> DHSLEAQWTKWKAMHNRLYGMNEEGWRRAVWEK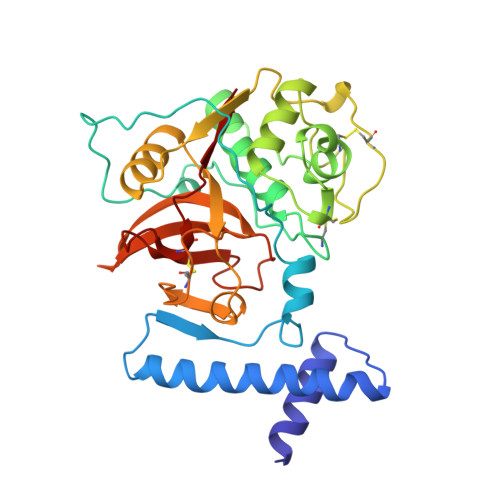NMKMIELHNQEYREGKHSFTMAMNAFGDMTSEEFRQVMNGLQNRKPRKGKVFQEPLFYEAPRSVDWREKGYVTPVKNQGQCGSSWAFSATGALEGQMFRKTGRLISLSEQNLVDCSGPEGNEGCNGGLMDYAFQYVQDNGGLDSEESYPYEATEESCKYNPKYSVANDAGFVDIPKQEKALMKAVATVGPISVAIDAGHESFLFYKEGIYFEPDCSSEDMDHGVLVVGYGFESTESDGNKYWLVKNSWGEEWGMGGYVKMAKDRRNHCGIASAASYPTV> DNATPLGKATFVLKNDNDKSETSHETVEGSGEATFENIKPGDYTLREETAPIGYKKTDKTWKVKVADNGATIIEGMDADKAEKRKEVLNAQYPKSAIYEDTKENYPLVNVEGSKVGEQYKALNPINGKDGRREIAEGWLSKKITGVNDLDKNKYKIELTVEGKTTVETKELNQPLDVVVLLDNSNSMNNERANNSQRALKAGEAVEKLIDKITSNKDNRVALVTYASTIFDGTEATVSKGVADQNGK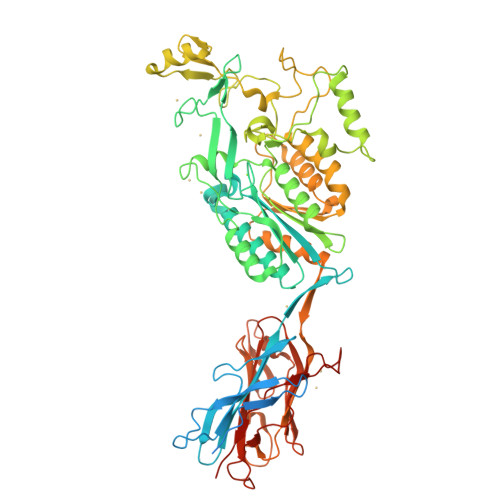ALNDSVSWDYHKTTFTATTHNYSYLNLTNDANEVNILKSRIPKEAEHINGDRTLYQFGATFTQKALMKANEILETQSSNARKKLIFHVTDGVPTMSYAINFNPYISTSYQNQFNSFLNKIPDRSGILQEDFIINGDDYQIVKGDGESFKLFSDRKVPVTGGTTQAAYRVPQNQLSVMSNEGYAINSGYIYLYWRDYNWVYPFDPKTKKVSATKQIKTHGEPTTLYFNGNIRPKGYDIFTVGIGVNGDPGATPLEAEKFMQSISSKTENYTNVDDTNKIYDELNKYFKTIVEEKHSIVDGNVTDPMGEMIEFQLKNGQSFTHDDYVLVGNDGSQLKNGVALGGPNSDGGILKDVTVTYDKTSQTIKINHLNLGSGQKVVLTYDVRLKDNYISNKFYNTNNRTTLSPKSEKEPNTIRDFPIPKIRDVREFPVLTISN> XYEKPALPRK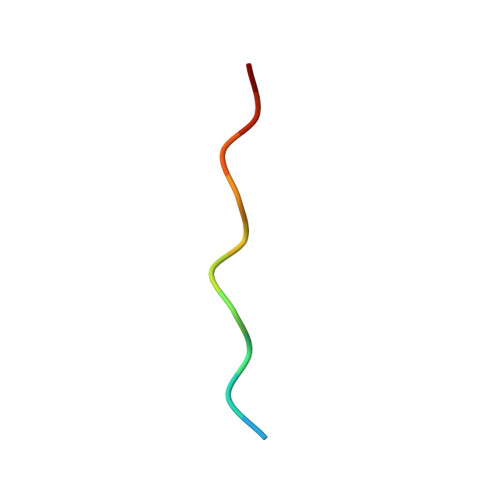RX> GSHNGIDCSFWNESYLTGSRDERKKSLLSKFGMDEGVTFMFIGRFDRGQKGVDVLLKAIEILSSKKEFQEMRFIIIGKGDPELEGWARSLEEKHGNVKVIT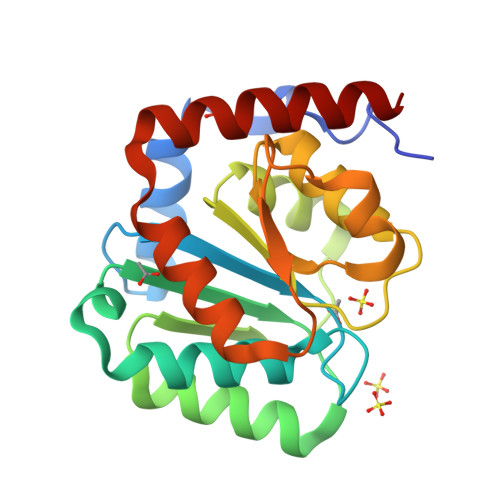EMLSREFVRELYGSVDFVIIPSYFEPFGLVALEAMCLGAIPIASAVGGLRDIITNETGILVKAGDPGELANAILKALELSRSDLSKFRENCKKRAMSFS>[2x]SAFDQAARSRGHSNRRTALRPRRQQEATEVRPEQKMPTLL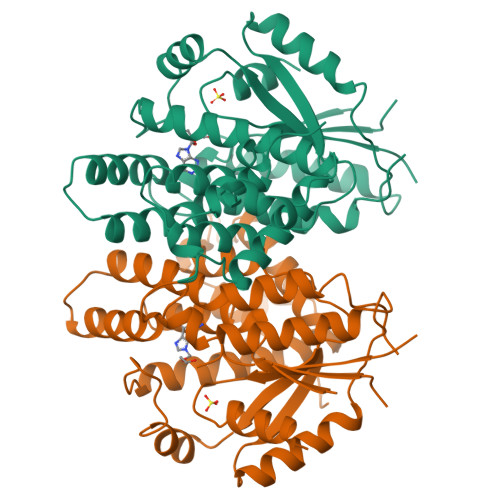RVYIDGPHGMGKTTTTQLLVALGSRDDIVYVPEPMTYWRVLGASETIANIYTTQHRLDQGEISAGDAAVVMTSAQITMGMPYAVTDAVLAPHIGGEAGSSHAPPPALTLIFDRHPIAALLCYPAARYLMGSMTPQAVLAFVALIPPTLPGTNIVLGALPEDRHIDRLAKRQRPGERLDLAMLAAIRRVYGLLANTVRYLQCGGSWREDWGQLSGTAVPPQGAEPQSNAGPRPHIGDTLFTLFRAPELLAPNGDLYNVFAWALDVLAKRLRSMHVFILDYDQSPAGCRDALLQLTSGMVQTHVTTPGSIPTICDLARTFAREMGEAN>QIVTDNSIGNHDGYDYEFWKDSGGSGTMILNHGGTFSAQWNNVNNILFRKGKKFNETQTHQQVGNMSINYGANFQPNGNAYLCVYGWTVDPLVEYYIVDSWGNWRPPGATPKGTITVDGGTYDIYETLRVNQPSIKGIATFKQYWSVRRSKRTSG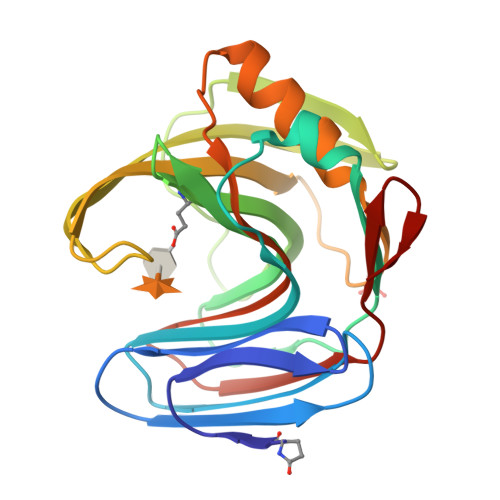TISVSNHFRAWENLGMNMGKMYEVALTVEGYQSSGSANVYSNTLRINGNPLS[2x]>[4x]MSLTIKLIAIDIDGTLLNEKNELAQATIDAVQAAKAQGIKVVLCTGRPLTGVQPYLDAMDIDGDDQYAITFNGSVAQTISGKVLTNHSLTYEDYIDLEAWARKVRAHFQIETPDYIYTANKDISAYTIAESYLVR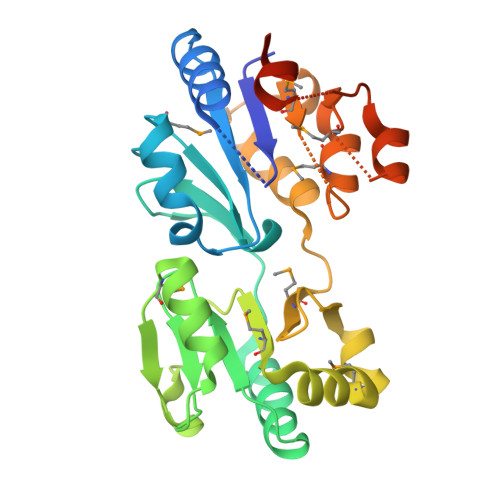MLIQYREVSETPRDLTISKAMFVDYPQVIEQVKANMPQDFKDRFSVVQSAPYFIEVMNRRASKGGTLSELVDQLGLTADDVMTLGDQGNDLTMIKYAGLGVAMGNAIDEVKEAAQAVTLTNAENGVAAAIRKYALNEGHHHHHH>MTKKGDTYNEAWVKDTNGFDILMGQFAHNIENIWGFKEVVIAGPKDYVKYTD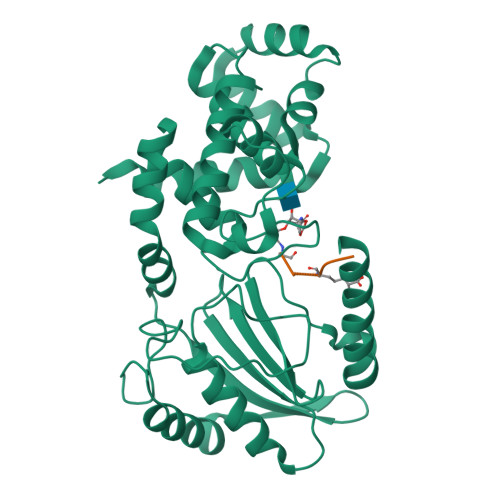QYQTRSHINFDDGTITIETIAGTEPAAHLRRAIIKTLLMGDDPSSVDLYSDVDDITISKEPFLYGQVVDNTGQPIRWEGRASNFADYLLKNRLKSRSNGLRIIYSVTINMVPNHLDKRAHKYLGMVRQASRKYGVDESLILAIMQTQSSFNPYAVSRSDALGLMQVVQHTAGKDVFRSQGKSGTPSRSFLFDPASNIDTGTAYLAMLNNVYLGGIDNPTSRRYAVITAYNGGAGSVLRVFSNDKIQAANIINTMTPGDVYQTLTTRHPSAESRRYLYKVNTAQKSYRRR[2x];> AEKAA2-fluoranyl-5-[2-[4-(4-methyl-1,2,4-triazol-3-yl)piperidin-1-yl]pyridin-3-yl]pyridine 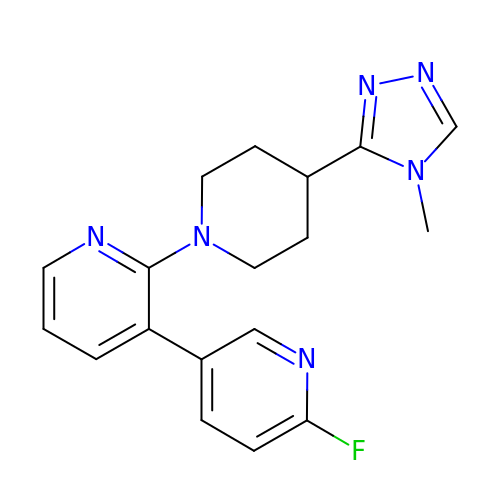| C18 H19 F N6 | AJIAMIPUWJQSPR-UHFFFAOYSA-N> MQWETVIGLEIHAQLATQSKIFSGSSTAFGAAPNTQASLVDLAMPGTLPVLNEEAVRMACLFGLAIDARIDRQNVFARKNYFYPDLPKGYQTSQMDHPIVGKGH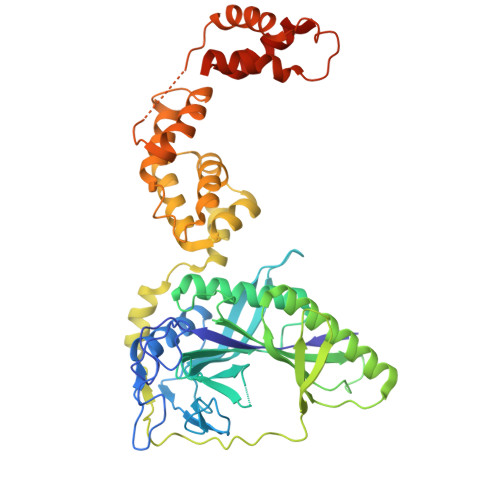LDITLEDGTTKRIGITRAHLEEDAGKSLHEDFQGMSGIDLNRAGTPLLEIVSEPDIRSAKEAVAYVKAIHALVRYLGICDGNMAEGSLRCDCNVSVRPKGQAEFGTRAEIKNVNSFRFIEKAINHEIQRQIELIEDGGKVVQETRLYDPNKDETRSMRGKEEANDYRYFPCPDLLPVVIEPEYLAKLREQLPELPVQKRERFESQYGLSAYDASVLSASREMADYFEKVQGICGDAKLAANWVMVELGSLLNKDGLEIEQSPVSAEQLGGMILRIKDNTISGKLAKMVFEAMANGEGSAXXXXXXXXXXXXXXXXXXXXXXXXXXXXXXXXXXXXXXXXXXXXXXXXXXXXXXXXXXXXXXXXXXXXXXXXXXXXXX>SNAMRNKNMSTIYQTSATASAGRNGVVSTEDKLLELNLSYPKEMGGSGTATNPEQLFAVGYAACFSNAILHVARE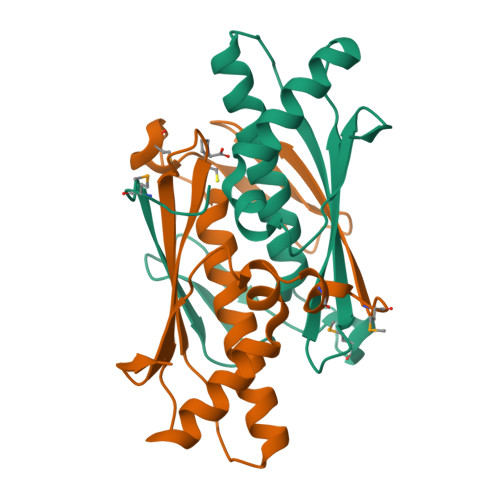AKVALKEAPVTATVGIGPNGQGGFALSVALAAHIALEDEQARQLVTVAHQVCPYSNAVRGNIDVQVSVNGLAL[2x]> GSHGGIEGVKGAASGVVGELARARLALDERGQKLSDLEERTAAMMSSADSFSKHAHEMMLKYK;> GSHSKQALSEIETRHSEIIKLENSIRELHDMFMDMAMLVESQGEMIDRIEYNVEHAVDYVERAVSDTKKAVKYQS;> GSHMRNELEEMQRRADQLADESLESTRRMLQLVEESK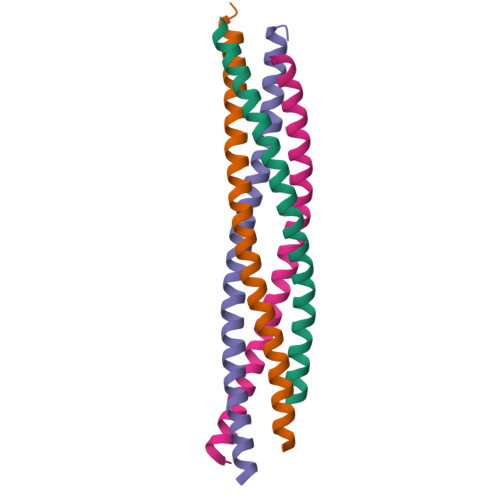DAGIRTLVMLDEQGEQLDRVEEGMNHINQDMKEAEKNLKDLGK;> GSHMASRENEMDENLEQVSGIIGNLRHMALDMGNEIDTQNRQIDRIMEKADSNKTRIDEANQRATKMLG> MGGSHHHHHHGENLYFQSVDDLTVEPNLHSLITSTTHKWIFVGGKGGVGKTTSSCSIAIQMALSQPNKQFLLISTDPAHNLSDAFGEKFGKDARKVTGMNNLS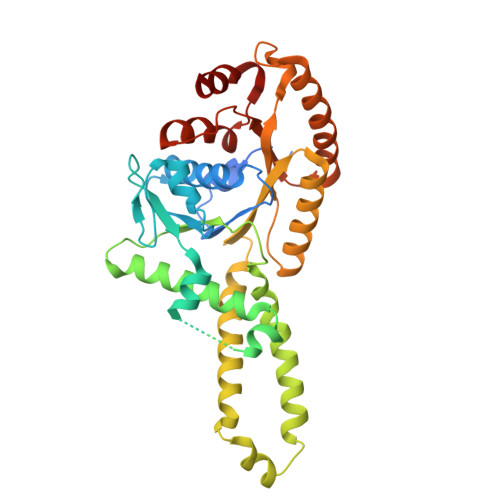CMEIDPSAALKDMNDMAVSRANNNGSDGQGDDLGSLLQGGALADLTGSIPGIDEALSFMEVMKHIKRQEQGEGETFDTVIFDTAPTGHTLRFLQLPNTLSKLLEKFGEITNKLGPMLNSFMGAGNVDISGKLNELKANVETIRQQFTDPDLTTFVCVCISEFLSLYETERLIQELISYDMDVNSIIVNQLLFAENDQEHNCKRCQARWKMQKKYLDQIDELYEDFHVVKMPLCAGEIRGLNNLTKFSQFLNKEYNPITDGKVIYELEDKE4-{[4-(dimethylamino)butanoyl]amino}-N-(3-{[4-(pyridin-3-yl)pyrimidin-2-yl]amino}phenyl)benzamide 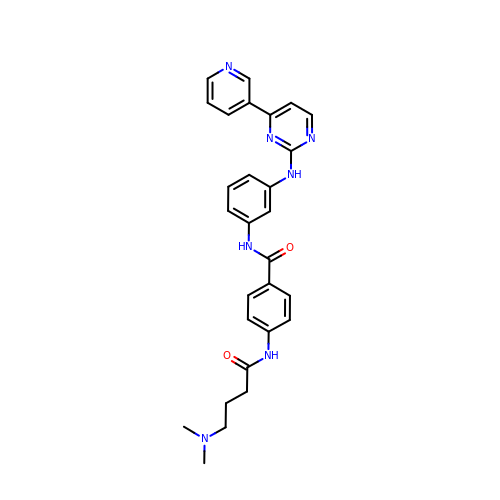| C28 H29 N7 O2 | UHHXMHJPSLUZFX-UHFFFAOYSA-N>MRILVVNVNTTASITETIAEQARAVASPGTEIVGLTPYFGAESVEGNFESYLAAIAVMDRVMAYDQPFDAVIQAGYGEHGREGLQELLNVPVVDITEAAASTAMFLGHAYSVVTTLDRTVPLIEDRLKLAGLYQRCASVRASGMAVLELEEDPVAAMEAIVRQAELAIREDKAEVICLGCGGMAGLDEQIRQRTGVPVV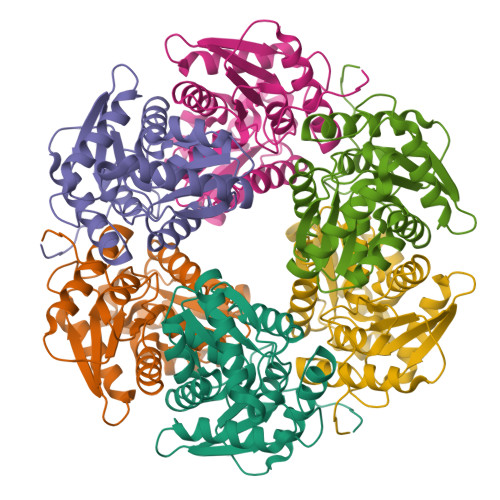DGVTAAVTIAESLVRLGLSTSKIRTYATPRPKKVIGWPGRLGR[2x]> MGSDKIHHHHHHENLYFQGMIRLGKMSDLDQILNLVEEAKELMKEHDNEQWDDQYPLLEHFEEDIAKDYLYVLEENDKIYGFIVVDQDQAEWYDDIDWPVNREGAFVIHRLTGSKEYKGAATELFNYVIDVVKARGAEVILTDTFALNKPAQGLFAKFGFHK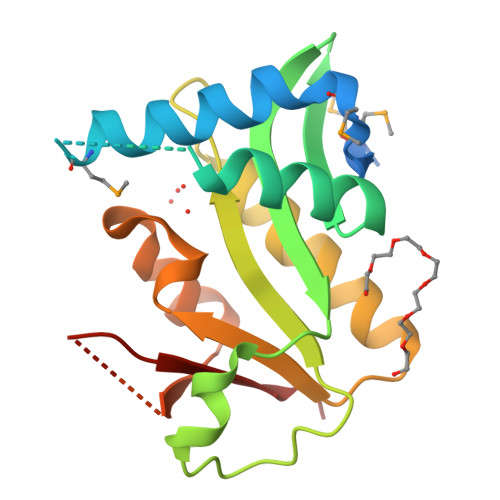VGEQLMEYPPYDKGEPFYAYYKNLKE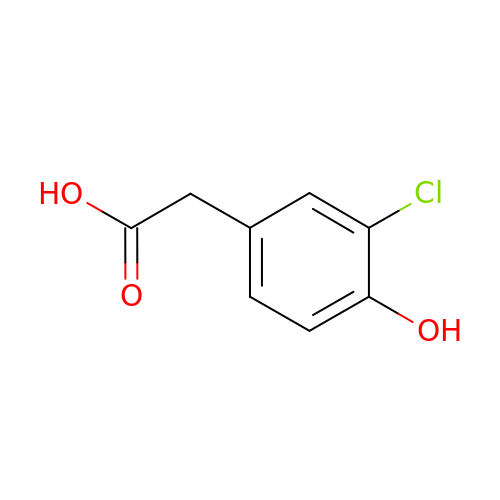(3-CHLORO-4-HYDROXYPHENYL)ACETIC ACID | C8 H7 Cl O3 | IYTUKSIOQKTZEG-UHFFFAOYSA-N A paradigmatic example for a drug target with a transient binding pocket is the FK506 binding protein 51 (FKBP51), encoded by the FKBP5 gene. FKBP51 is an intracellular protein belonging to the immunophilin family. Like many other members of the FKBPs family, it has a peptidyl-prolyl isomerase (PPIase) activity, can act as a co-chaperone of heat shock protein 90 (Hsp90) and it plays a role in the regulation of steroid hormone receptor activity. In humans, FKBP51 is linked to several stress-related disorders (e.g., anxiety disorders or depression), obesity, type 2 diabetes, and chronic pain.

The iFit ligand class (including its analogs SAFit-FL and SAFit1) were the first molecules capable of selectively inhibiting FKBP51. The binding of these ligands stabilizes a conformational change in the FKBP51 FK1 domain. This conformational change is characterized by the displacement of the F67 side chain which creates a transient-binding pocket to accommodate the iFit ligands. As the G64S variant showed the strongest improvements in the binding affinity of both FKBP51-selective ligands and its role in the formation of the transient binding pocket is not obvious, we decided to explore the molecular basis for the binding affinity enhancement in more detail. With a Kd of 0.09 ± 0.01 nM for SAFit-FL (out/in) and 0.7 ± 0.2 nM for Mcyc-TA (out/out), the affinity of this variant showed a 10- and 34-fold increase, respectively, while no improvement of ligand binding was seen for the canonical inhibitor FK [431]-TA (in/in) 3. Interestingly, for none of the three ligands a direct interaction between the ligand and the newly introduced serine 64 can be observed. In the FKBP51-G64S:SAFit1 (out/in) complex the loop involving serine 64 is slightly shifted and S64 engages in a hydrogen bond with K60. For the binding of SAFit-FL (out/in) only a serine substitution on position 64 shows a strong improvement in binding affinity. Strikingly, in the SAFit1-bound state S64 forms a hydrogen bond with the side chain of lysine 60, which seems not to be possible for the other G64 variants. Taken together, our results for the FKBP51-G64 variants strongly suggest that the improvement of the binding affinity of our conformation-specific ligands is due to a combination of destabilization of unproductive protein conformations, augmented for very favorable cases by specific stabilization of the productive conformation, and not due to novel contacts with the ligand.

> GAPATVTEQGEDITSKKDRGVLKIVKRVGNGEETPMIGDKVYVHYKGKLSNSKKFDSSHDRNEPFVFSLGKGQVIKAWDIGVATMKKGEIAHLLIKPEYAYGSAGSLPKIPSNATLFFEIELLDFKGE>[4x]MDYKDDDDKERDVLEREFQRVTISGEEKCGVPFTDLLDAAKSVVRALFIREKYMALSLQSFCPTTRRYLQQLAEKPLETRTYEQGPDTPVSADAPVHPPALEQHPYEHCEPSTMPGDLGLGLRMVRGVVHVYTRREPDEHCSEVELPYPDLQEFVADVNVLMALIINGPIKSFCYRRLQYLSSKFQMHVLLNEMKELAAQKKVPHRDFYNIRKVDTHIHASSCMNQKHLLRFIKRAMKRHLEEIVHVEQGREQTLREVFESMNLTAYDLSVDTLDVHADRNTFHRFDKFNAKYNPIGESVLREIFIKTDNRVSGKYFAHIIKEVMSDLEESKYQNAELRLSIYGRSRDEWDKLARWAVMHRVHSPNVRWLVQVPRLFDVYRTK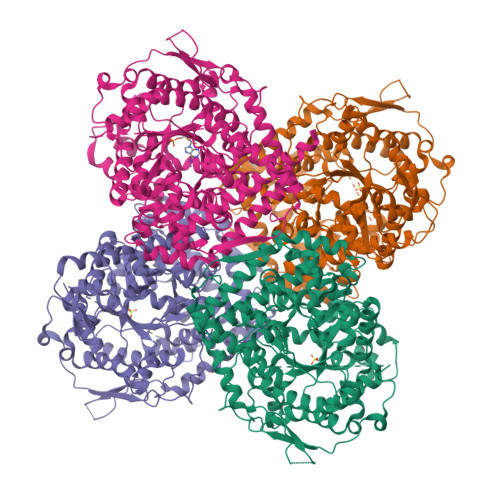GQLANFQEMLENIFLPLFEATVHPASHPELHLFLEHVDGFDSVDDESKPENHVFNLESPLPEAWVEEDNPPYAYYLYYTFANMAMLNHLRRQRGFHTFVLRPHCGEAGPIHHLVSAFMLAENISHGLLLRKAPVLQYLYYLAQIGIAMSPLSNNSLFLSYHRNPLPEYLSRGLMVSLSTDDPLQFHFTKEPLMEEYSIATQVWKLSSCDMCELARNSVLMSGFSHKVKSHWLGPNYTKEGPEGNDIRRTNVPDIRVGYRYETLCQELALITQAVQSEMLETIPEEAGITMSPGPQ> AKTPVIVVPVIDRLPSETFPNVHEHINDQKFDDVKDNEVMPEKRNVVVVKDDPDHYKDYAFIQWTGGNIRNDDKYTHFFSGFCNTMCTEETKRNIARHLALWDSNFFTELENKKVEYVVIVENDNVIEDITFLRPVLKAMHDKKIDILQMREIITG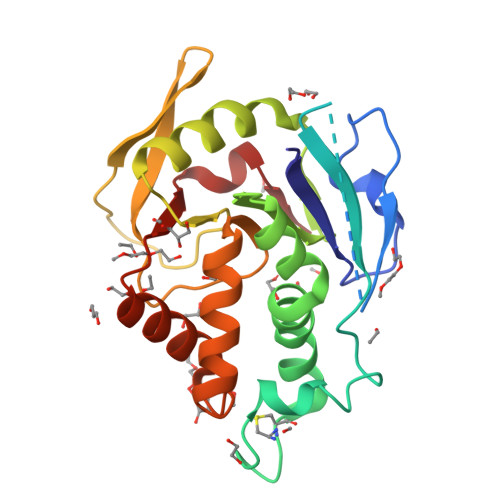NKVKTELVMDKNHAIFTYTGGYDVSLSAYIIRVTTALNIVDEIIKSGGLSSGFYFEIARIENEMKINRQILDNAAKYVEHD> ALTGSRPSVVYLHAAECTGCSEALLRTYQPFIDTLILDTISLDYHETIMAAAGEAAEEALQAAVNGPDGFICLVEGAIPTGMDNKYGYIAGHTMYDICKNILPKAKAVVSIGTCACYGGIQAAKPNPTAAKGINDCYADLGVKAINVPGCPPNPLNMVGTLVAFLKGQKIELDEVGRPVMFFGQSVHDLCERRKHFDAGEFAPSFNSEEARKGWCLYDVGCKGPET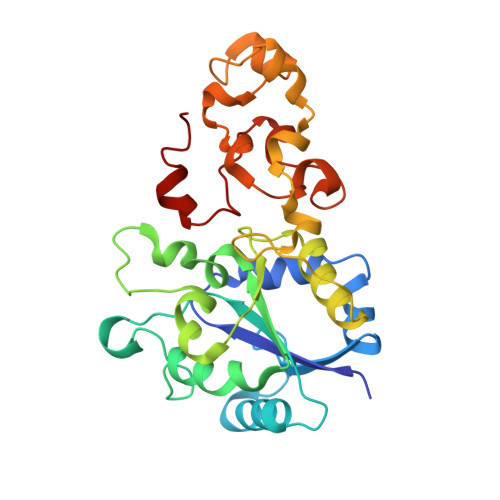YNNCPKVLFNETNWPVAAGHPCIGCSEPNFWDDMTPFYQN> GDPVEDIIHDALGSTARRAISSATNVESAANTTPSSHRLETGRVPALQAAETGATSNATDENMIETRCVVNRNGVLETTINHF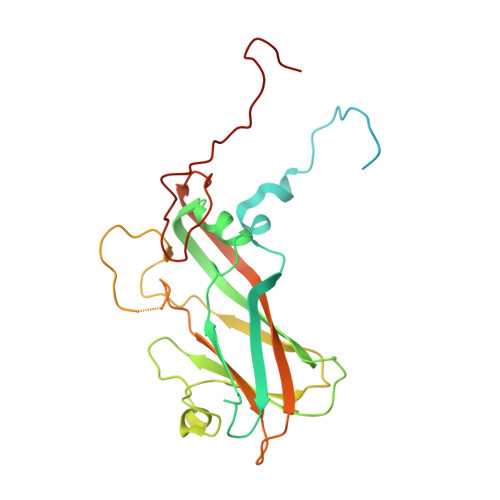FSRSGLVGVVNLTDGGTDTTGYVTWDIDIMGFVQLRRKCEMFTYMRFNAEFTFVTTTKNGEARPYMLQYMYVPPGAPKPTGRDAFQWQTATNPSVFVKLTDPPAQVSVPFMSPASAYQWFYDGYPTFGQHPETSNTTYGLCPNNMMGTFAVRVVSREASQLKLQTRVYMKLKHVRAWVPRPIRSQPYLLKNFPNYDSSKITNSARDRSSIKQANM1-{[2-(difluoromethoxy)phenyl]methyl}-2,2-dimethyl-1,2-dihydro-3H-indol-3-one 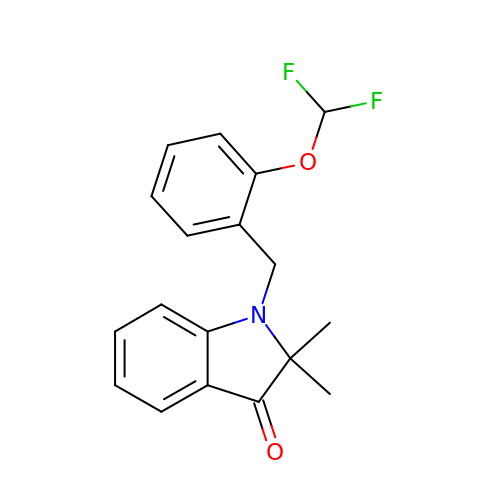| C18 H17 F2 N O2 | BSVSFPVFEQPRJW-UHFFFAOYSA-N EV-D68 is an atypical enterovirus that usually causes mild respiratory tract disease, but is also associated with severe lower respiratory tract infections and acute flaccid myelitis. Following receptor binding and endocytosis, virus particles uncoat by forming a proteinaceous pore spanning the endosomal membrane through which they eject their genome into the cytosol. In this study, we showed that EV-D68-947 is a dual receptor-binding virus that can use both sialylated glycans and sGAGs as receptors. Structures of EV-D68-947 were determined after incubation of the virus either in the absence of a receptor analogue, with 6′SLN (a sialylated trisaccharide), with dp6 (a heparin-derived hexasaccharide), or with LMWH at 33 °C.

Full and empty particles in cryo-EM images were counted. e Structure of EV-D68-947 empty capsids formed in the absence or presence of LMWH. VP2 residues 53–60, 98–100, and 240–242 and VP3 residues 148–150, which line the hole around the two-fold axis, are less ordered in emptied particles formed after LMWH treatment than in those formed without ligand. Incubation of EV-D68-947 with sGAG analogues not only caused pocket factor displacement but also promoted genome release, by enlarging the putative openings for genome egress at the two-fold axes via a yet unknown mechanism.

> IESIIKTATDTVKSEINAELGVVPSLNAVETGATSNTEPEEAIQTRTVINQHGVSETLVENFLSRAALVSKRSFEYKDHTSSAAQTDKNFFKWTINTRSFVQLRRKLELFTYLRFDAEITILTTVAVNGSSNNTYMGLPNLTLQAMFVPTGALTPEKQDSFHWQSGSNASVFFKISDPPARMTIPFMCINSAYSVFYDGFAGFEKSGLYGINPADTIGNLCVRIVNEHQPVGFTVTVRVYMKPKHIKAWAPRPPRTLPYMSIANANYKGKKRAPNALNAIIGNRDSVKTMPHNIVTT;> GVPTYLLPGSGQFLTTDDHSSAPVLPCFNPTPEMHIPGQVRNMLEVVQVESMMEINNTESAVGMERLKVDISALTDVDQLLFNIPLDIQLDGPLRNTLVGNISRYYTHWSGSLEMTFMFCGSFMATGKLILCYTPPGGSCPTTRETAMLGTHIVWDFGLQSSVTLIIPWISGSHYRMFNNDAKSTNANVGYVTCFMQTNLIVPSESSDTCSLIGFIAAKDDFSLRLMRDSPDIGQIDHLHAAEAAYQ;> SPSAEACGYSDRVLQLKLGNSAIVTQEAANYCCAYGEWPNYLPDHEAVAIDKPTQPETATDRFYTLKSVKWEAGSTGWWWKLPDALNNIGMFGQNVQHHYLYRSGFLIHVQCNATRFHQGALLVVAIPEHQRGAHNTNTSPGFDDIMKGEEGGTFNHPYVLDDGTSLACATIFPHQWINLRTNNSATIVLPWMNAAPMDFPLRHNQWTLAIIPVVPLGTRTMSSMVPITVSIAPMCCEFNGLRHAITQ(2R)-N-(3-{[(2H-1,3-benzodioxol-5-yl)methyl]amino}-3-oxopropyl)-2-hydroxy-3,3-dimethylbutanamide | C17 H24 N2 O5 | 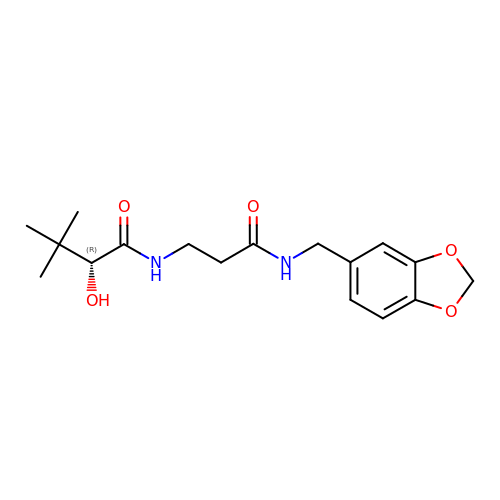CABNSQJZPOAZEV-HNNXBMFYSA-N The HD transcription factor WUS plays key roles for plant development with at least four distinct and essential subfunctions: Firstly, regulation of stem cell identity in the shoot apical meristem (SAM), where it is required for non cell-autonomous induction and maintenance of stem cell fate via stimulation of cytokinin and suppression of auxin signaling. Consistent with a broad functional portfolio, WUS has been shown to bind to a diverse set of DNA motifs in the regulatory regions of downstream genes involved in SAM development and signaling processes. Here, we have combined molecular, biochemical, and structural approaches to address how the WUS-HD recognizes specific DNA target sites. We find that the DNA-binding preferences of WUS-HD depend on appropriately arranged sequence motifs in a direct tandem repeat and that homodimerization is one of the key determinants to achieve high sequence specificity.

To elucidate the structural basis for these differential interactions, we solved crystal structures of WUS-HD bound to TAAT, G-Box and TGAA repeat probes to resolutions of 2.8, 2.7 and 1.6 Å, respectively. Intriguingly, the TGAA repeat probe was bound by WUS-HD with much higher affinity (Kd = 0.27 ± 0.03 µM; ± indicates standard deviation, n = 3) than the other two sequences. Interestingly, in the case of G-Box and TAAT, one of the two protein–DNA complexes in the asymmetric unit contained an additional bound HD, whereas both TGAA structures only included two HDs per DNA. In contrast, the two HD molecules interacting with the TAAT and the TGAA repeat probes were on opposite sides of the DNA and formed specific protein-protein modifications between each other. One of the WUS-HD molecules bound to the TGAA probe made additional DNA contacts through stabilization of the helix α3 C-terminus by the other WUS molecule, which might explain the higher affinity for the TGAA sequence. In particular, R96 and R100 of the recognition helix established new contacts to the DNA-backbone, not observed in any of the other WUS–DNA complexes. Notably, in the case of the TGAA homodimer, which showed the highest binding affinity, the HDs associate non-symmetrically via the C-terminal end of the recognition helix (α3), thereby establishing additional contacts with the DNA. In contrast, in the TGAA structure A93 contacted the thymine from the complementary strand, which base paired with the adenine of the +1 position. Interestingly, the affinity of an ideal 2xTGAA DNA repeat was similar to that of the naturally occurring TGAA repeat probe from the CLV1 locus (Kd = 0.27 ± 0.03 µM; ± indicates standard deviation, n = 3), suggesting the binding of two WUS-HD molecules per DNA as seen in our TGAA crystal structure.

>[4x]GAMGQTSTRWTPTTEQIKILKELYYNNAIRSPTADQIQKITARLRQFGKIEGKNVFYWFQNHKARERQKKRFNGGS The coronavirus spike protein (S protein), an envelope-anchored trimeric type I transmembrane glycoprotein, mediates receptor binding and the fusion of the viral and host cell membranes, which is treated as the main target of neutralizing antibodies and vaccine development. The S protein is composed of two subunits, the N-terminal S1 subunit containing the N-terminal domain (NTD) and receptor-binding domain (RBD), which are responsible for binding cellular receptors (sugars and proteins), and the C-terminal S2 subunit possessing a fusion peptide (FP), two heptad repeats (HR) and a transmembrane domain, which drives membrane fusion by undergoing a large conformational rearrangement. Here, we report the cryo-EM structures of the HCoV-229E S trimers with two conformations, named conformation 1 and 2, at resolutions of 3.21 and 3.55 Å, respectively. Our structures illustrate the dynamic conformational changes that occur in the prefusion states of Alphacoronavirus S trimers, providing a better understanding of the molecular mechanisms underlying receptor binding and the transition from pre- to postfusion.

After further data processing, we finally identified two major conformational states: conformation 1 (derived from peak 2) and conformation 2 (derived from peak 3) with resolutions of 3.21 and 3.55 Å, respectively. The C1 presents a slender conformation with a total of ~145 Å long and ~113 Å wide, while the C2 is a stubby structure with ~132 Å long and ~117 Å wide, which is ~13 Å shorter than C1 and the shortest among the S protein structures reported previously. Meanwhile, we observed that the interaction interface between protomers decreased from C1 to C2 (with average interaction interfaces of ~4824 and ~4145 Å2 for C1 and C2, respectively). In addition, through analysis of the C1 density map, there are 31 sugar molecules identified on the surface of the S protein, most of which are located in the S1 subunit. The RBD (chain A) interacts with the NTD (chain A) and the adjacent NTD (chain C), RBD (chain C), and RBD (chain B). This interactional mode between the NTDs and RBDs may cause the RBDs in C1 to remain in a lying state. In the C1 state, S1-RBDs are buried through their interactions with the surrounding S1-NTDs and S1-RBDs in the same or adjacent protomer and are not available for binding to hAPN. Specifically, the equilibrium dissociation constant (KD) of peak 2 and hAPN is 36.3 ± 0.071 nM, and of peak 3 and hAPN is 6.78 ± 0.105 nM. First, the inaccessible closed state (C1) can transform to an activated state1 (C2), which reduces the steric conflicts for RBD transformation to the “standing” state.

>MFVLLVAYALLHIAGCQTTNGLNTSYSVCNGCVGYSENVFAVESGGYIPSDFAFNNWFLLTNTSSVVDGVVRSFQPLLLNCLWSVSGLRFTTGFVYFNGTGRGDCKGFSSDVLSDVIRYNLNFEENLRRGTILFKTSYGVVVFYCTNNTLVSGDAHIPFGTVLGNFYCFVNTTIGNETTSAFVGALPKTVREFVISRTGHFYINGYRYFTLGNVEAVNFNVTTAETTDFCTVALASYADVLVNVSQTSIANIIYCNSVINRLRCDQLSFDVPDGFYSTSPIQSVELPVSIVSLPVYHKHTFIVLYVDFKPQSGGGKCFNCYPAGVNITLANFNETKGPLCVDTSHFTTKYVAVYANVGRWSASINTGNCPFSFGKVNNFVKFGSVCFSLKDIPGGCAMPIVANWAYSKYYTIGSLYVSWSDGDGITGVPQPVEGVSSFMNVTLDKCTKYNIYDVSGVGVIRVSNDTFLNGITYTSTSGNLLGFKDVTKGTIYSITPCNPPDQLVVYQQAVVGAMLSENFTSYGFSNVVELPKFFYASNGTYNCTDAVLTYSSFGVCADGSIIAVQPRNVSYDSVSAIVTANLSIPSNWTTSVQVEYLQITSTPIVVDCSTYVCNGNVRCVELLKQYTSACKTIEDALRNSAMLESADVSEMLTFDKKAFTLANVSSFGDYNLSSVIPSLPRSGSRVAGRSAIEDILFSKLVTSGLGTVDADYKKCTKGLSIADLACAQYYNGIMVLPGVADAERMAMYTGSLIGGIALGGLTSAASIPFSLAIQSRLNYVALQTDVLQENQKILAASFNKAMTNIVDAFTGVNDAITQTSQALQTVATALNKIQDVVNQQGNSLNHLTSQLRQNFQAISSSIQAIYDRLDIIQADQQVDRLITGRLAALNVFVSHTLTKYTEVRASRQLAQQKVNECVKSQSKRYGFCGNGTHIFSLVNAAPEGLVFLHTVLLPTQYKDVEAWSGLCVDGRNGYVLRQPNLALYKEGNYYRITSRIMFEPRIPTIADFVQIENCNVTFVNISRSELQTIVPEYIDVNKTLQELSYKLPNYTVPDLVVEQYNQTILNLTSEISTLENKSAELNYTVQKLQTLIDNINSTLVDLKWLNRVETYIKWPW[3x]> GTCCTACCTGGCAGGACGACT;> ACACCGATCACCTGCCACCGTGTCTA;> TCTGATGTG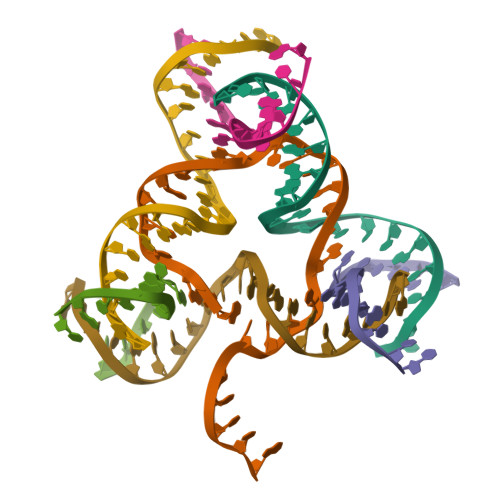GTAGG;> ACAGTCGTGGTATC;> TGCGTAGTGGTCGC;> CAGATACCTGATCGGACTACG;> GAGCGACCTGTACGGACATCA> GSQKERLLDELTLEGVARYMQSQRCRRVICLVGAGISTSAGIPDFRSPSTGLYDNLEKYHLPYPEAIFEISYFKKHPEPFFALAKEL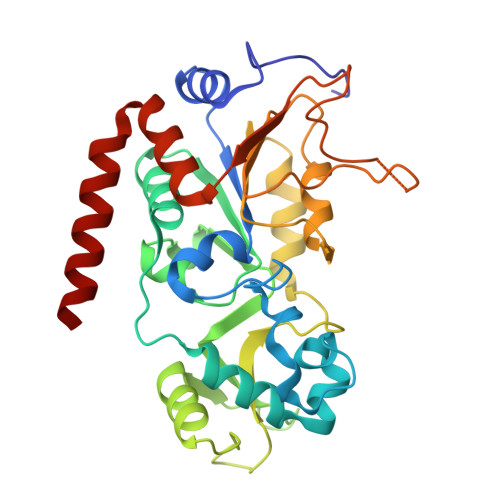YPGQFKPTICHYFMRLLKDKGLLLRCYTQNIDTLERIAGLEQEDLVEAHGTFYTSHCVSASCRHEYPLSWMKEKIFSEVTPKCEDCQSLVKPDIVFFGESLPARFFSCMQSDFLKVDLLLVMGTSLQVQPFASLISKAPLSTPRLLINKEKAGQSDPFLGMIMGLGGGMDFDSKKAYRDVAWLGECDQGCLALAELLGWKKELEDLVRREHASIDAQ> GAMGPLEEAIKDVDVSGVLRYRYDTGNFDKNFLNNSNLNNSKQDHKYRAQVNFSAAIADNFKAFVQFDYNAVDGGTGVDNATNAEKGLFVRQLYLTYTNEDVAT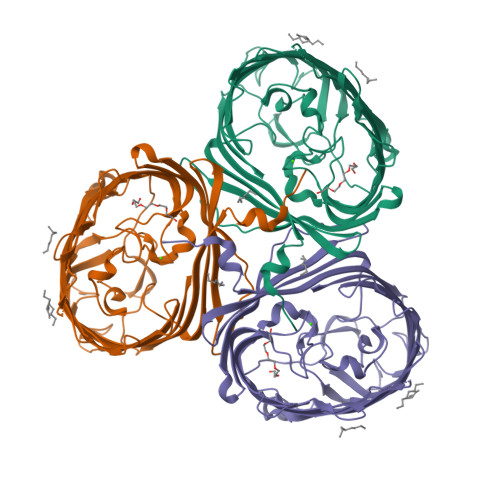SVIAGKQQLNIIWTDNGVDGLVGTGVKVVNNSIDGLTLAAFAVDSFMAAEQGSDLLGQSTYVGNGKNNNDSFKLDSIGNLYGAAAVGSYDLAGGQFNPQLWLAYWDQVAFFYAVDAAYSTTIFDGINWTLEGAYLGNSLDSELDDKKTYANGNLFALKGSIEVNGWDASLGGLYYGDKEKASTVVIEDQGNLGSLLAGEEIFYTTGSRLNGDTGRNIFGYVTGGYTFNETVRVGADFVYGGTKTEATTHLGGGKKLEAVARVDYKYSPKLNFSAFYSYVNLDQGVNTNESADHSTVRLQALYKF> MLGNFRFDDMVEKLSRRVAGRTSRRGAIGRLGTVLAGAALVPLLPVDRRGRVSRANAAGPAEGVDPRAKWQPQDNDIQACDYWRHCSIDGNICDCSGGSLTNCPPGTKLATASWVASCYNPTDGQSYLIAYRDCCG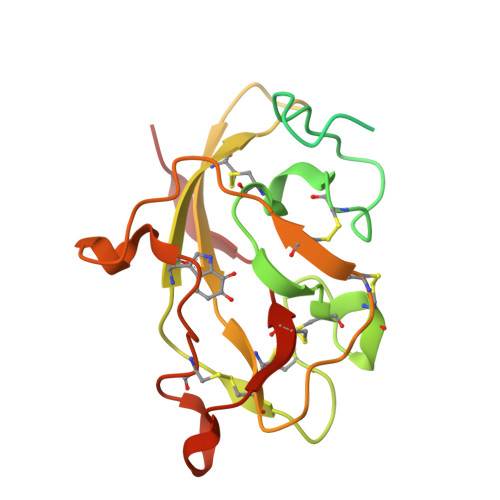YNVSGRCPCLNTEGELPVYRPEFANDIIWCFGAEDDAMTYHCTISPIVGKAS>GTSTQTKAGSLTIVGTGIESIGQMTLQALSYIEAAAKVFYCVIDPATEAFILTKNKNCVDLYQYYDNGKSRLNTFTQMSELMVREVRKGLDVVGVFYGHPGVFVNPSHRALAIAKSEGYRARMLPGVSAEDCLFADLCIDPSNPGCLTYEASDFLIRDRPVSIHSHLVLFQVGCVGIADFNFTGFDNNKFGVLVDRLEQEYGAEHPVVHYIAAMMPHQDPVTDKYTVAQLREPEIAKRVGGVSTFYIPPKARKASNLDIIRRLELLPAGQVPDKKARIYPANQWEPDVPEVEPYRPSDQAAIAQLADHAPPEQYQPLATSKAMSDVMTKLALDPKALADYKADHRAFAQSVPDLTPQERAALELGDSWAIRCAMKNMPSSLLDAARESGEEASQNGFPWVI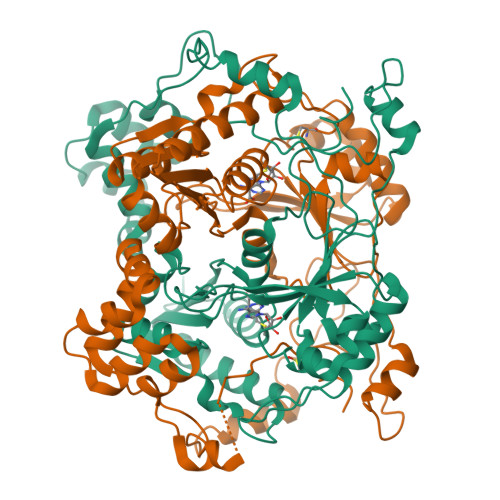VVGVIGVIG[2x]>SNAMIIRDENYFTDKYELTRTHSEVLEAVKVVKPGKTLDLGCGNGRNSLYLAANGYDVDAWDKNAMSIANVERIKSIENLDNLHTRVVDLNNLTFDGEYDFILSTVVLMFLEAKTIPGLIANMQRCTKPGGYNLIVAAMDTADYPCTVGFPFAF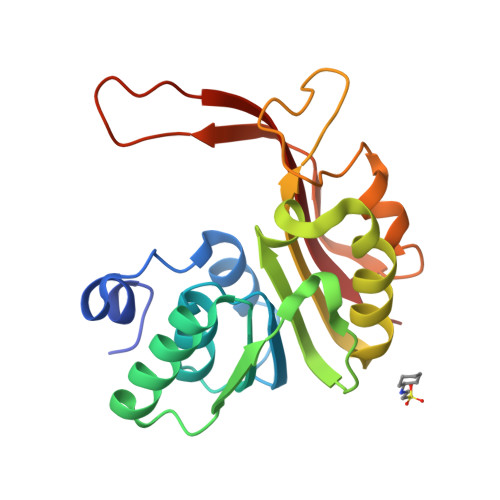KEGELRRYYEGWEMVKYNEDVGELHRTDANGNRIKLRFATMLARKK[4x]> HHAADYVLYKDATKPVEDRVADLLGRMTLAEKIGQMTQIERLVATPDVLRDNFIGSLLSGGGSVPRKGATAKEWQDMVDGFQKACMSTRLGIPMIYGIDAVHGQNNVYGATIFPHNVGLGATRDPYLVKRIGEATALEVRATGIQYAFAPCIAVCRDPRWGRCYESYSEDRRIVQSMTELIPGLQGDVPKDFTSGMPFVAGKNKVAACAKHFVGDGGTVDGINENNTIINREGLMNIHMPAYKNAMDKGVSTVMISYSSWNGVKMHANQDLVTGYLKDTLKFKGFVISDWEGIDRITTPAGSDYSYSVKASILAGLDMIMVPNKYQQFISILTGHVNGGVIPMSRIDDAVTRILRVKFTMGLFENPYADPAMAEQLGKQEHRDLAREAARKSLVLLKNGKTSTDAPLLPLPKKAPKILVAGSHADNLGYQCGGWTIEYQGDTGRTTVGTTILEAVKAAVDPSTVVVFAENPDAEFVKSGGFSYAIVAVGEHPYTETKGDNLNLTIPEPGLSTVQAVCGGVRCATVLISGRPVVVQPLLAASDALVAAWLPGSEGQGVTDALFGDFGFTGRLPRTWFKSVDQLPMNVGDAHYDPLFRLGYGLTTNATKKY

In the barley β-d-glucan glucohydrolase, a glycoside hydrolase family 3 (GH3) enzyme, the Trp286/Trp434 clamp ensures β-d-glucosides binding, which is fundamental for substrate hydrolysis during plant growth and development. HvExoI folds into a two-domain structure consisting of an (α/β)8 barrel (domain 1) and an (α/β)6 sandwich (domain 2) with a 13 Å-deep active site pocket embracing the subsites −1 and +1, positioned at the interface between the two domains. HvExoI catalyses the hydrolytic removal of nonreducing glucose (Glc) moiety from a broad spectrum of poly- and oligomeric β-d-glucosides. The crucial role of substrate binding in HvExoI implies a pair of the aromatic Trp286 and Trp434 residues that form a clamp at the +1 subsite, which is positioned next to a pocket-shaped site at the −1 subsite, housing the Asp285 and Glu491 catalysts.

On the other hand, in W286F the electron density map of G2SG-OMe was defined at the −1 and +1 subsites, where this thio-ligand formed H-bonds with Asp95, Lys206, His207, Arg158, Tyr253, Asp285, Arg291, and Glu491, and stacking interactions with W286F and Trp434, whereas G2SG-OMe did not bind to W286A and W286Y. The dispositions of G2SG-OMe at the −1 and +1 subsites in the W434A, W434F, W434H, and W434Y mutants revealed similar structural features of the ligand binding to those seen in W286F. Notable was the behaviour of W286Y that showed increased catalytic efficiency values with (1,3;1,6)-β-d-glucan (laminarin), laminaribiose (G3OG), and 4NP-Glc, while these values in W434Y were considerably lower.>[2x]EAKPSGSVVEQAEGVECD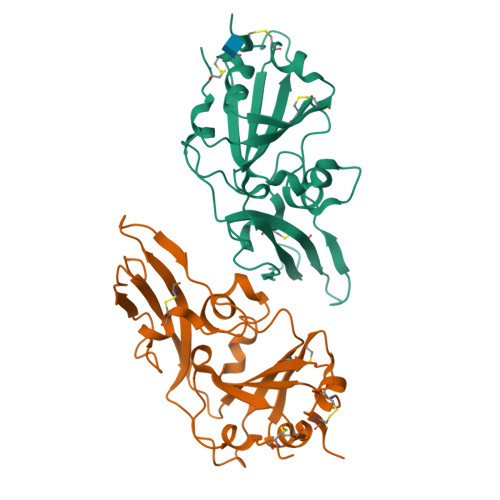FSPLLSGTPPQVYNFKRLVFTNCNYNLTKLLSLFSVNDFTCSQISPAAIASNCYSSLILDYFSYPLSMKSDLSVSSAGPISQFNYKQSFSNPTCLILATVPHNLTTITKPLKYSYINKCSRLLSDDRTEVPQLVNANQYSPCVSIVPSTVWEDGDYYRKQLSPLEGGGWLVASGSTVAMTEQLQMGFGITVQYGTDTNSVCPKLEFANDTKIASQLGNCVEYHHHHHH>HMASMTGGQQMGRGSRRSEKSRVAIVEATRALLLERGFDGLSIEAVAAKAGVGKQTIYRWWPSRHALVADVLLEDADKILARMPKTDDVTADLASWAGTLAAALTTRRGHAMLKTLMAASLEHEDTAARLR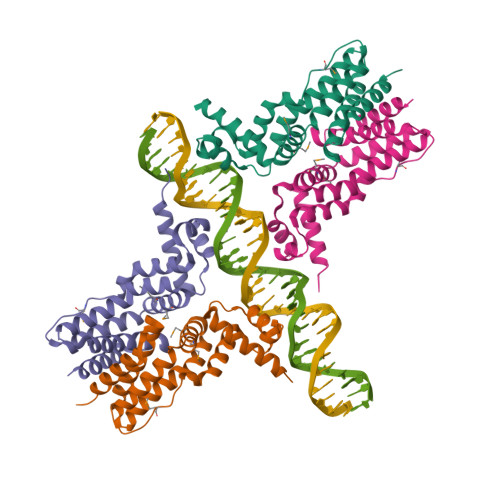EGFSRPLIESVRDRLRDEDIDADHAQAAADALLGAVVNAVLSEGRSYSRQRAETSARIIVAGLRP[4x]N-(furan-2-ylmethyl)quinoxaline-6-carboxamide | C14 H11 N3 O2 | 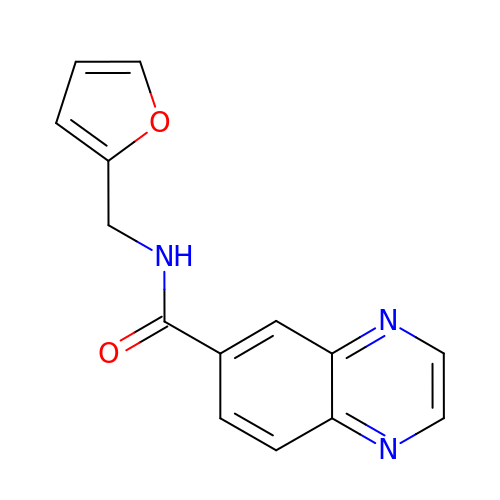HNDVFGAJLBLXDW-UHFFFAOYSA-N> G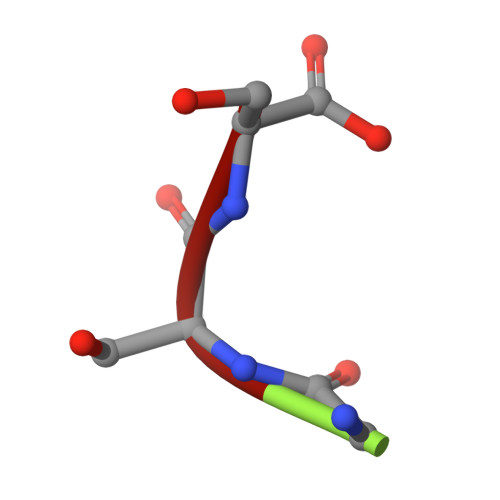SS>[2x]LVPAGSHMMKTLSLQSRAKTTALKQPKEIFAFARDIDGEFVYDQKIVKDENVSYYYLPDSKIDGSIDLQAGYAKFKKIPEEKNMSDMKCLLTALTKYEQEHNNGEKVNVDIITYRGLMTKLLALPYNLNDPVDLNVLAYDGQLFINSDEEIELARRKEEDEHKQQSMTPEKYDHMKRCEFSGYKFEAIATLPKPWADCSRQQIDKRGKKMVNNYEQYISVIKTGIGEAKMLLAGEVDCVWDYIPEDGKDVLSHYMELKTTRILESNGQVVNFEKKLFKTWAQCFLMGIRKVVYGFRDDSFFLRDVELYKTEEIPLLIKNNALTENKSGGKINCTTALKWYGAVIEWLLQEIPRDDTSKAYRVSFDPSTRTFTLRELMGNENSRLRNGEMLTSEFKQWRESIQK

Rai1 homologs share several highly conserved sequence motifs, and our structural studies show that they are located in the active site region, mediating the binding of the divalent metal ions and/or the RNA. We have found substantial variations in the activity profiles of the Rai1 homologs, and discovered that some of them possess a new 5′ triphosphonucleotide hydrolase (TPH) activity. The overall structures of CaRai1, AgRai1 and SsRai1 are similar to those of SpRai1 (16), KlDxo1 (18), and MmDXO. Each structure contains two mixed β-sheets that are surrounded by α-helices.

The CaRai1 and SsRai1 structures are especially similar, consistent with the 58% sequence identity between them. The αC helix is absent in AgRai1 but contains more than four turns in CaRai1 and SsRai1, which also have a longer αD helix. Therefore, AgRai1, CgRai1 and SsRai1 have a distinct 5′ triphosphonucleotide hydrolase (TPH) activity and do not have PPH activity. AgRai1 again showed strong activity, while consistently weaker activity was observed for SsRai1. At the same time, there are substantial differences in the positions of the helices, the connecting loops and even some of the β-strands among some of the structures, and these differences are especially pronounced for the β4-αA loop, αC and αD helices and the connecting loop, which form one wall of the active site pocket.>TFAGDNGTMMQYFEWYLPNDGTLWTKMGSDASHLKSIGITGVWFPPAYKGQSQSDVGYGVYDMYDLGEFNQKGTVRTKYGTKAQLQSAITSLHNNGIQAYGDVVLNHRMGADATETISAVEVNPSNRNQVTSGAYNISAWTDFEFPGRGNTYSSFKWHSYYFDGVDWDQSRQLSGKIYQIQGKAWDWEVDSENGNYDYLMGADIDYDHPDVQTEVKNWGKWFVNTLNLDGVRLDAVKHIKFDYMSSWLSSVKSTTGKSNLFAVGEYWNTSLGALENYENKTNWSMSLFDVPL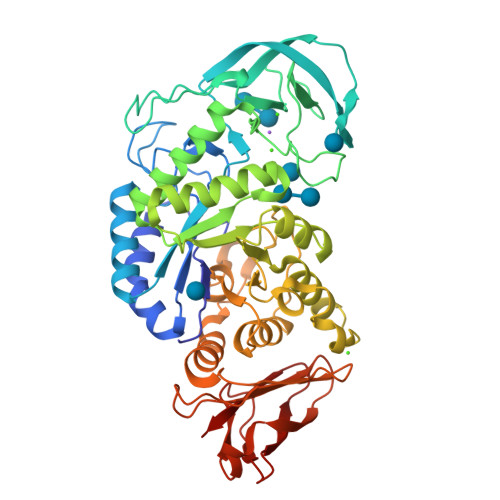HMNFQAAANGGGYYDMRNLLNNTMMKNHPIQAVTFVDNHDTEPGQALQSWVSDWFKPLAYATILTRQEGYPCVFYGDYYGIPSQSVSAKSTWLDKQLSARKSYAYGTQHDYLDNQDVIGWTREGDSAHAGSGLATVMSDGPGGSKTMYVGTAHAGQVFKDITGNRTDTVTINSAGNGTFPCNGGSVSIWVKQ[4x]>[2x]MNISDVAKITGLTSKAIRFYEEKGLVTPPMRSENGYRTYTQQHLNELTLLRQA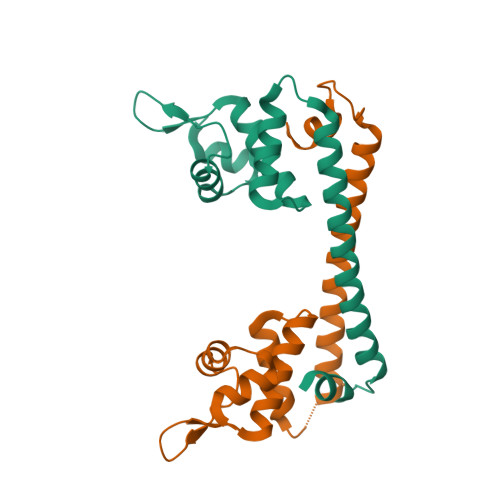RQVGFNLEESGELVNLFNDPQRHSADVKRRTLEKVAEIERHIEELQSMRDQLLALANACPGDDSADCPIIENLSGCCHHRAG>MGLSINPTLINRDKPYTKEELMEILRLAIIAELDAINLYEQMARYSEDENVRKILLDVAREEKAHVGEFMALLLNLDPEQVTELKGGFEEVKE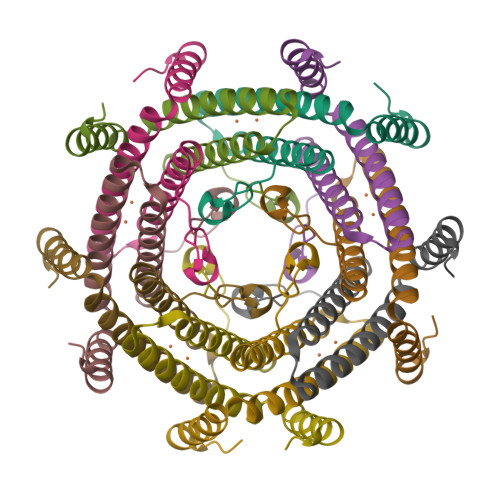LTGIEA[30x]>ETLLGFYKQYKALSEYIDKKYKLSLNDLAVLDLTMKHCKDEKVLMQSFLKTAMDELDLSRTKLLVSIRRLIEKERLSKVRSSKDERKIYIYLNNDDISKFNALFEDVEQFLNILEHHHHHH[2x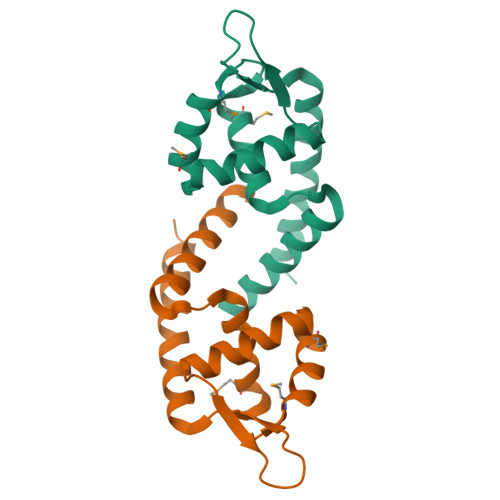]>MARKYFVAANWKCNGTLESIKSLTNSFNNLDFDPSKLDVVVFPVSVHYDHTRKLLQSKFSTGIQNVSKFGNGSYTGEVSAEIAKDLNIEYVIIGHFDRRKYFHETDEDVREKLQASLKNNLKAVVCFGESLEQREQNKTIEVITKQVKAFVDLIDNFDNVILVYEPLWAIGTGKTATPEQAQLVHKEIRKIVKDTCGEKQANQIRI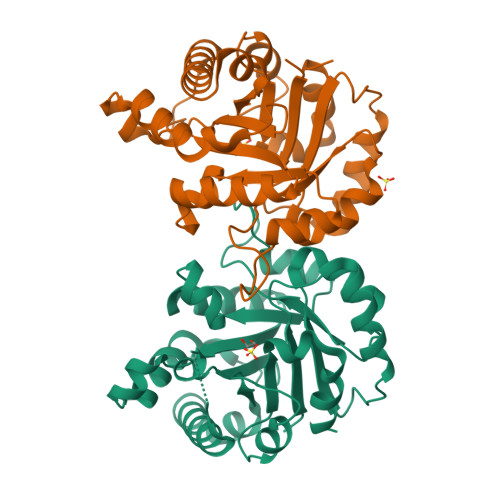LYGGSVNTENCSSLIQQEDIDGFLVGNASLKESFVDIIKSAM[2x]>[5x]MSEQTIYGANTPGGSGPRTKIRTHHLQRWKADGHKWAMLTAYDYSTARIFDEAGIPVLLVGDSAANVVYGYDTTVPISIDELIPLVRGVVRGAPHALVVADLPFGSYEAGPTAALAAATRFLKDGGAHAVKLEGGERVAEQIACLTAAGIPVMAHIGFTPQSVNTLGGFRVQGRGDAAEQTIADAIAVAEAGAFAVVMEMVPAELATQITGKLTIPTVG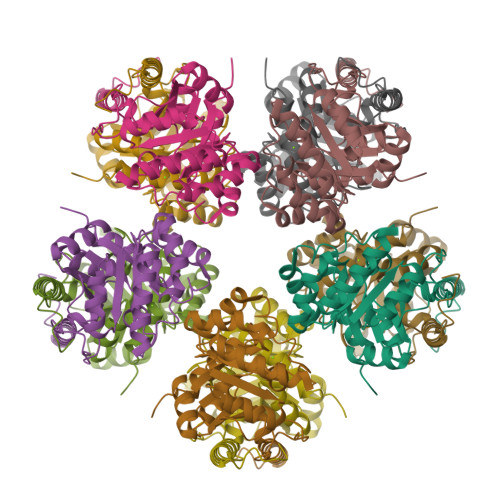IGAGPNCDGQVLVWQDMAGFSGAKTARFVKRYADVGGELRRAAMQYAQEVAGGVFPADEHSF6-chloranyl-3-[(dimethylamino)methyl]-4~{H}-pyrrolo[1,2-a]quinazolin-5-one 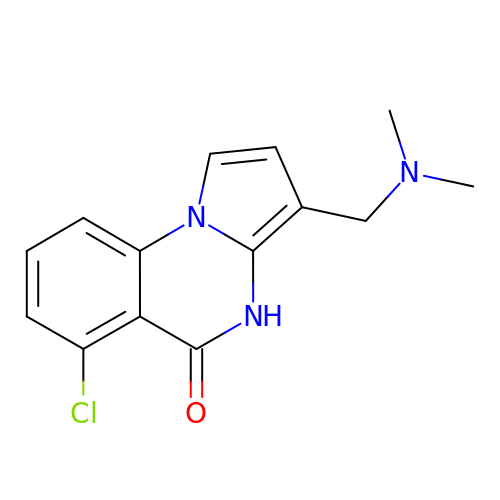| C14 H14 Cl N3 O | FSTYDISPXAAJMK-UHFFFAOYSA-N>HTLYAPGGYDIMGYLIQIMNRPNPQVELGPVDTSCALILCDLKQKDTPIVYASEAFLYMTGYSNAEVLGRNCRFLQSPDGMVKPKSTRKYVDSNTINTIRKAIDRNAEVQVEVVNFK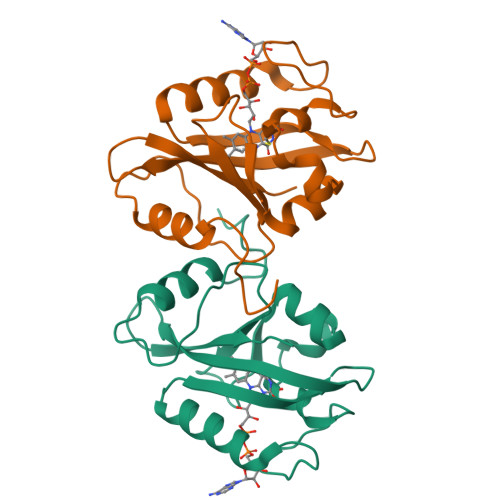KNGQRFVNFLTIIPVRDETGEYRYSMGFQCE[2x]>MNYPVNPDLMPALMAVFQHVRTRIQSELDCQRLDLTPPDVHVLKLIDEQRGLNLQDLGRQMCRDKALITRKIRELEGRNLVRRERNPSDQRSFQLFLTDEGLAIHQHAEAIMSRVHDELFAPLTPVEQATLVHLLDQSLAA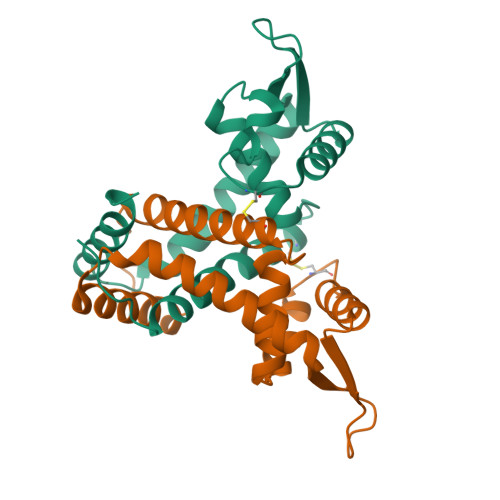Q[2x]> MSYYHHHHHHEGVRTMDSKYQCVKLNDGHFMPVLGFGTYAPAEVPKSKALEATKLAIEAGFRHIDSAHLYNNEEQVGLAIRSKIADGSVKREDIFY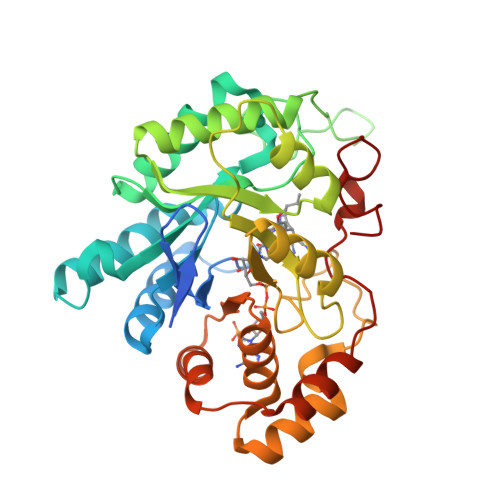TSKLWCNSHRPELVRPALERSLKNLQLDYVDLYLIHFPVSVKPGEEVIPKDENGKILFDTVDLCATWEAVEKCKDAGLAKSIGVSNFNRRQLEMILNKPGLKYKPVCNQVECHPYFNQRKLLDFCKSKDIVLVAYSALGSHREEPWVDPNSPVLLEDPVLCALAKKHKRTPALIALRYQLQRGVVVLAKSYNEQRIRQNVQVFEFQLTSEEMKAIDGLNRNVRYLTLDIFAGPPNYPFSDEY> GHKPEPTDEEWELIKTVTEAHVATNAQGSHWKQKRKFLPEDIGQAPIVNAPEGGKVDLEAFSHFTKIITPAITRVVDFAKKLPMFCELPCEDQIILLKGCCMEIMSLRAAVRYDPESETLTLNGEMAVTRGQLKNGGLGVVSD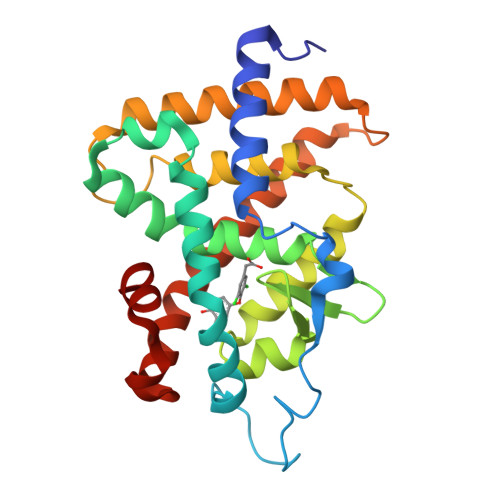AIFDLGMSLSSFNLDDTEVALLQAVLLMSSDRPGLACVERIEKYQDSFLLAFEHYINYRKHHVTHFWPKLLMKVTDLRMIGACHASRFLHMKVECPTELFPPLFLEVFE>GSVVIVGRII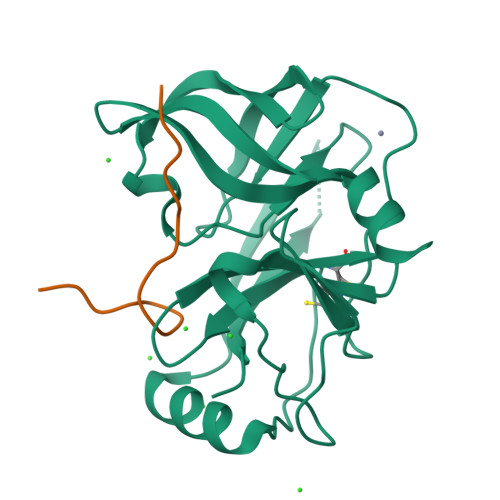LSGKGGPITAYSQQTRGLLGCIITSLTGRDRNQVEGEVQVVSTATQSFLATCVNGVCWTVYHGAGSKTLAGPKGPITQMYTNVDQDLVGWQAPPGARSLTPCTCGSSDLYLVTRHADVIPVRRRGDSRGSLLSPRPVSYLKGSSGGPLLCPSGHAVGIFRAAVCTRGVAKAVDFVPVESMETTMRGSHHHHHH[2x];>[2x]GELGRLVYLLDGPGYDPIHCD Connexin family proteins assemble into hexameric channels called hemichannels/connexons, which function as transmembrane channels or dock together to form gap junction intercellular channels (GJIChs). Human Cx31.3/GJC3, which is expressed in oligodendrocytes of the central nervous systems, does not form intercellular channels. We determined the cryo–electron microscopy structures of human connexin 31.3 (Cx31.3)/GJC3 hemichannels in the presence and absence of calcium ions and with a hearing-loss mutation R15G at 2.3-, 2.5-, and 2.6-Å resolutions, respectively. We also found that the hemichannel has a pore with a diameter of ~8 Å and selectively transports chloride ions.

Two mutations R15G and L23H in human Cx31.3 have been found to cause nonsyndromic hearing loss, and biochemical study in HeLa cells demonstrated that these mutations inhibit ATP release through Cx31.3 hemichannel. To confirm the ATP transport activity of Cx31.3 hemichannel and the inhibitory effect of R15G mutation, we performed the ATP release assay using purified hemichannels. The result showed that wild-type proteoliposomes, mutant proteoliposomes, and protein-free liposomes retained ~100, ~500, and ~500 pmol of ATPs, respectively. This indicates that wild-type proteoliposomes released most ATPs during the desalting process, while mutant proteoliposomes retained ATPs in the similar level as free liposomes. Compared with the wild-type hemichannel structure, the R15G mutant showed some changes in the polar interaction network between NTH and TM2 and notably decreased the basicity of the cytoplasmic surface. However, we found no major structural change and almost no change in the pore diameter at the cytoplasmic entrance by this mutation. This, together with the ATP transport assay, suggests that ATP molecules cannot freely diffuse through the mutant hemichannel in the entrance-covering NTH conformation. Because the pore diameter (~8 Å) at the cytoplasmic entrance is much smaller than the effective hydrated diameter of ATP (~12 Å), this conformation would not allow ATP to move through the pore without substantial conformational changes of NTHs. The hemichannel structure showed that the entrance-covering NTH conformation forms a small pore slightly bigger than hydrated K+ or Cl− ions, suggesting that the transport of metabolites much bigger than ions would require a conformational change of NTH. This idea is further supported by the ATP-impermeable R15G-mutant hemichannel structure that also adopts a similar NTH conformation. However, it is still unclear how the wild-type hemichannel, but not the mutant, could change the NTH conformation to transport ATP.

>MCGRFLRRLLAEESGRSTPVGRLLLPVLLGFRLVLLAASGPGVYGDEQSEFVCHTQQPGCKAACFDAFHPLSPLRFWVFQVILVAVPSALYMGFTLYHVIWHWELSGKGKEEETLIQGREGNTDVPGAGSLRLLWAYVAQLGARLVLEGAALGLQYHLYGFQMPSSFACRREPCLGSITCNLSRPSEKTIFLKTMFGVSGFCLLFTFLELVLLGLGRWWRTWKHKSSSSKYFLTSESTRRHKKATDSLPVVETKEQFQEAVPGRSLAQEKQRPVGPRDA[6x]>NLKPVDAMQCFDCHTQIEDMHTVGKHATVNCVHCHDATEHVETASSRRMGERPVTRMDLEACATCHTAQFNSFVEVRHESHPRLEKATPTSRSPMFDKLIAGHGFAFEHAEPRSHAFMLVDHFVVDRAYGGRFQFKNWQKVTDGMGAVRGAWTVLTDADPESSDQRRFLSQTATAANPVCLNCKTQDHILDWAYMGDEHEAAKWSRTSEVVEFARDLNHPLNCFMCHDPHSAGPRVVRDGLINAVVDRGLGTYPHDPVKSEQQGMTKVTFQRGREDFRAIGLLDTADSNVMCAQCHVEYNCNPGYQLSDGSRVGMDDRRANHFFWANVFDYKEAAQEIDFFDFRHATTGAALPKLQHPEAETFWGSVHERNGVACADCHMPKVQLENGKVYTSHSQRTPRDMMGQACLNCHAEWTEDQALYAIDYIKNYTHGKIVKSEYWLAKMIDLFPVAKRAGVSEDVLNQAR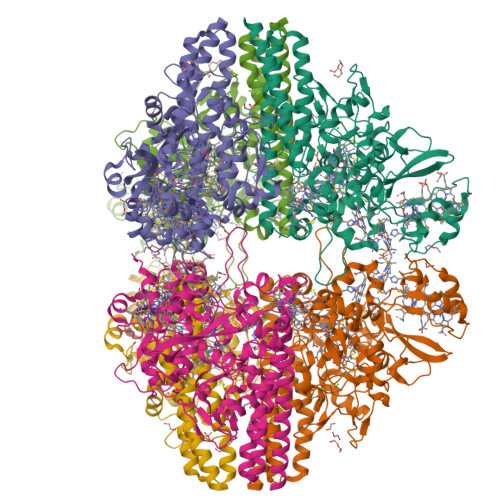ELHYDAHLYWEWWTAENSVGFHNPDQARESLMTSISKSKEAVSLLNDAIDAQVA[2x]>[2x]MSAIKPDMKIKLRMEGNVNGHHFVIDGDGTGKPFEGKQSMDLEVKEGGPLPFAFDILTTAFAYGNRVFAKYPDNIQDYFKQSFPKGYSWERSLTFEDGGICNARNDITMEGDTFYNKVRFYGTNFPANGPVMQKKTLKWEPSTEKMYVRDGVLTGDVETALLLEGNAHYRCDFRTTYKAKEKGVKLPGAHFVDHCIEILSHDKDYNKVKLYEHAVAHSGLPN

The system studied was a reversibly switchable fluorescent protein (rsFP) which is a representative of a class of proteins that undergo a reversible photolysis reaction from a highly fluorescent “on” state to a weakly fluorescence “off” state. The specific rsFP used, rsKiiro, is a mutant of Skylan-NS33 specifically developed for ultrafast time-resolved crystallographic studies due to its ability to form crystals that diffract to high resolution (∼1.1 Å for single-crystal cryo-MX), high photoswitching quantum yield (∼18% Trans-to-Cis in the crystal), and high protein expression yields. Structurally, rsKiiro is similar to green fluorescent protein (GFP) with an 11-stranded β-barrel surrounding an α helix. The chromophore of rsKiiro is formed from the Ala-Tyr-Gly tripeptide at residue numbers 62–64 in the α helix.

In this study, we probed the light-induced reverse reaction, from the Trans to Cis chromophore conformation, initiated with 2 ms 405 nm pulses at a range of optical flash energy densities (0.1–6.7 mJ/mm2) after the initial Cis-to-Trans photoconversion had been driven to completion using ∼13 mW/mm2 of 473 nm CW illumination. A total of 435,200 images were obtained across 6 laser energy densities at 405 nm of 0, 0.1, 0.53, 1.78, 6.74, and 14.43 mJ/mm2. From these images, 79,976 single-crystal indexed diffraction patterns were obtained and merged into 6 data sets for each corresponding laser energy density. Data below a value of 0.5 in Fourier shell correlation were discarded, leading to a uniform limit of 1.7 Å being applied to all data sets. The initial examination of the chromophore-omitted maps clearly shows increasing occupancy of the Cis state at higher energy densities. A clear difference in reaction yield can be seen even when comparing the lowest flash energies (0.00 and 0.10 mJ/mm2), where a difference of 3% population transfer is determined from the shift in the minima.>[2x]SMDMPVERILEAELAVEPKTESYGDMNMENSTNDPVTNICHAADKQLFTLVEWAKRIPHFSDLTLEDQVILLRAGWNELLIASFSHRSVSVQDGILLATGLHVHRSSAHSAGVGSIFDRVLTELVSKMKDMQMDKSELGCLRAIVLFNPDAKGLSNPSEVETLREKVYATLEAYTKQKYPEQPGRFAKLLLRLPALRSIGLKCLEHLFFFKLIGDTPIDTFLMEMLETPLQIT;>KHKILHRLLQDSSY[2x]

The nuclear retinoid X receptor (RXR) is a unique family of ligand-activated transcription factors, which in humans comprises of three members, namely, RXRα (NR2B1), RXRβ (NR2B2) and RXRγ (NR2B3). All three RXR isoforms typically function as a universal heterodimer partner for other nuclear receptors, including the type II thyroid hormone receptors (THRs, NR1A1-2) and the peroxisome proliferator-activated receptors (PPARs, NR1C1-3). Here, we report a complete set of the crystal structures for all three RXR isoforms in active, ligand-bound conformation with an identical ligand. In addition, we discovered saturated fatty acids, including palmitic acid (PA), myristic acid (MA) and stearic acid (SA), as RXR modulators capable of inducing the recruitment of co-regulators to the RXR ligand-binding domain (LBD) and hence, activating the receptor.

We next questioned whether PA could also bind to the other two RXR isoforms and therefore, we crystallized and successfully determined the tertiary complex structures of both RXRβ and RXRγ with (exogenously added) PA and the GRIP-1 co-regulator peptide. The crystal structures indeed revealed the binding of PA to both isoforms in a similar manner to that observed for the alpha counterpart. These structures provided to our knowledge not only the first report of the ligand-bound RXRγ crystal structure, but a complete set of the same tertiary complexes of all three RXRs with an identical ligand. RXRα is mainly expressed in liver, kidney and spleen, while RXRβ is ubiquitously found and RXRγ expression is mostly limited to the CNS and muscles. RXRγ was particularly found to be involved in the regulation of CNS myelination, a key process in multiple sclerosis with high relevance also in Alzheimer’s disease (AD). To understand whether the 24 amino acid differences within the LBD region may have any indirect influence toward ligand-binding properties among the three isoforms, we mapped the differences onto the structures. We observed that although most changes were located peripherally at the surface of the proteins, there were three substitutions in the proximity of the ligand-binding pocket (site 3, site 11 and site 15 based on Figure 4a). Additionally, the amino acid change at site 3 with polar, aliphatic glutamine in the alpha and beta isoforms (Gln270 and Gln341, respectively) to basic, aromatic histidine (His271) in the gamma counterpart was particularly notable. This substitution could result in alterations of the protein properties, such as electrostatic charge, evident, for example, by a contact between helix 2 His271 and helix 12 Asp449 observed in the RXRγ structure, which was absent for the glutamine residues at the equivalent position in the other two isoforms.>MGSSHHHHHHENLYFQGCGHHQDSAKKESTSHKKKENDNEELNEELKEFKSKKNMDIKIKGDTIVSDKFEAKIKEPFIINEKDEKKKYIAFKMEITAKKDDKDLNPSSISHDYINITQDDKNTVNKLRDGYLLSDKKYKDWTEHNQDQIKKGKTAQAMFIYELRGDGNINLNVHKYSEDKTVDSKSFKFSKLKTEDFSHRAETR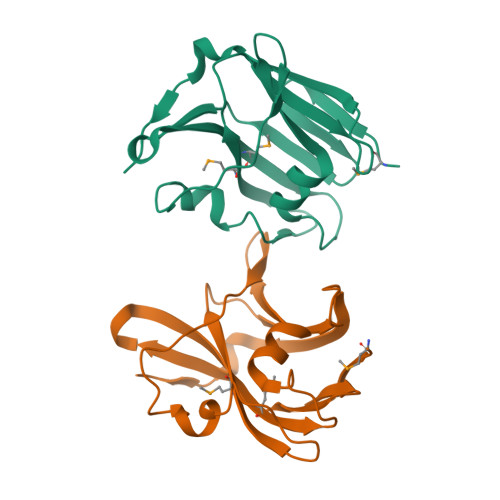EEVEKKEKEFEEEYKKEQEREKEKEKQKDDDHSGLDEV[2x]> MEPHVLGAGLYWLLLPCTLLAASLLRFNALSLVYLLFLLLLPWLPGPSRHSIPGHTGRLLRALLCLSLLFLVAHLAFQICLHTVPHLDQFLGQNGSLWVKVSQHIGVTRLDLKDIFNTTRLVAPDLGVLLASSLCLGLCGRLTRKAGQSRRTQELQDDDDDDDDDDEDIDAAPAVGLKGAPALATKRRLWLASRFRVTAHWLLMTSGRTLVIVLLALAGIAHPSAFSSIYLVVFLAICTWWSCHFPLSPLGFNTLCVMVSCFGAGHLICLYCYQTPFIQDMLPPGNIWARLFGLKNFVDLPNYSSPNALVLNTKHAWPIYVSPGILLLLYYTATSLLKLHKSCPSELRKETPREDEEHELELDHLEPEPQARDATQGEMPMTTEPDLDNCTVHVLTSQSPVRQRPVRPRLAELKEMSPLHGLGHLIMDQSYVCALIAMMVWSIMYHSWLTFVLLLWACLIWTVRSRHQLAMLCSPCILLYGLTLCCLRYVWAMELPELPTTLGPVSLHQLGLEHTRYPCLDLGAMLLYLLTFWLLLRQFVKEKLLKKQKVPAALLEVTVADTEPTQTQTLLRSLGELVTGIYVKYWIYVCAGMFIVVSFAGRLVVYKIVYMFLFLLCLTLFQVYYTLWRKLLRVFWWLVVAYTMLVLIAVYTFQFQDFPTYWRNLTGFTDEQLGDLGLEQFSVSELFSSILIPGFFLLACILQLHYFHRPFMQLTDLEHVPPPGTRHPRWAHRQDAVSEAPLLEHQEEEEVFREDGQSMDGPHQATQVPEGTASKWGLVADRLLDLAASFSAVLTRIQVFVRRLLELHVFKLVALYTVWVALKEVSVMNLLLVVLWAFALPYPRFRPMASCLSTVWTCIIIVCKMLYQLKIVNPHEYSSNCTEPFPNNTNLQPLEINQSLLYRGPVDPANWFGVRKGYPNLGYIQNHLQILLLLVFEAVVYRRQEHYRRQHQQAPLPAQAVCADGTRQRLDQDLLSCLKYFINFFFYKFGLEICFLMAVNVIGQRMNFMVILHGCWLVAILTRRRREAIARLWPNYCLFLTLFLLYQYLLCLGMPPALCIDYPWRWSKAIPMNSALIKWLYLPDFFRAPNSTNLISDFLLLLCASQQWQVFSAERTEEWQRMAGINTDHLEPLRGEPNPIPNFIHCRSYLDMLKVAVFRYLFWLVLVVVFVAGATRISIFGLGYLLACFYLLLFGTTLLQKDTRAQLVLWDCLILYNVTVIISKNMLSLLSCVFVEQMQSNFCWVIQLFSLVCTVKGYYDPKEMMTRDRDCLLPVEEAGIIWDSICFFFLLLQRRIFLSHYFLHVSADLKATALQASRGFALYNAANLKSINFHRQIEEKSLAQLKRQMKRIRAKQEKYRQSQASRGQLQSKDPQDPSQEPGPDSPGGSSPPRRQWWRPWLDHATVIHSGDYFLFESDSEEEEEALPEDPRPAAQSAFQMAYQAWVTNAQTVLRQRRERARQERAEQLASGGDLNPDVEPVDVPEDEMAGRSHMMQRVLSTMQFLWVLGQATVDGLTRWLRAFTKHHRTMSDVLCAERYLLTQELLRVGEVRRGVLDQLYVGEDEATLSGPVETRDGPSTASSGLGAEEPLSSMTDDTSSPLSTGYNTRSGSEEIVTDAGDLQAGTSLHGSQELLANARTRMRTASELLLDRRLHIPELEEAERFEAQQGRTLRLLRAGYQCVAAHSELLCYFIIILNHMVTASAASLVLPVLVFLWAMLTIPRPSKRFWMTAIVFTEVMVVTKYLFQFGFFPWNSYVVLRRYENKPYFPPRILGLEKTDSYIKYDLVQLMALFFHRSQLLCYGLWDHEEDRYPKDHCRSSVKDREAKEEPEAKLESQSETGTGHPKEPVLAGTPRDHIQGKGSIRSKDVIQDPPEDLKPRHTRHISIRFRRRKETPGPKGTAVMETEHEEGEGKETTERKRPRHTQEKSKFRERMKAAGRRLQSFCVSLAQ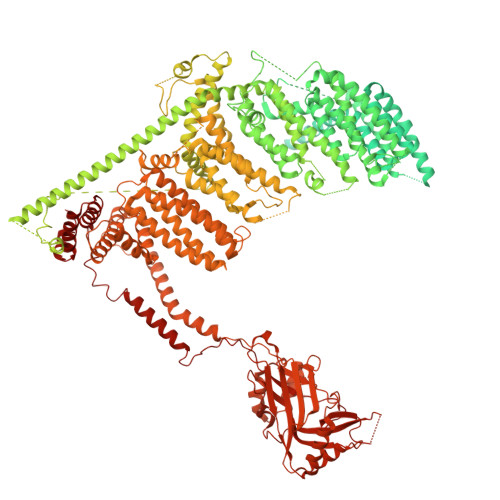SFYQPLQRFFHDILHTKYRAATDVYALMFLADIVDIIIIIFGFWAFGKHSAATDIASSLSDDQVPQAFLFMLLVQFGTMVIDRALYLRKTVLGKLAFQVVLVVAIHIWMFFILPAVTERMFSQNAVAQLWYFVKCIYFALSAYQIRCGYPTRILGNFLTKKYNHLNLFLFQGFRLVPFLVELRAVMDWVWTDTTLSLSNWMCVEDIYANIFIIKCSRETEKKYPQPKGQKKKKIVKYGMGGLIILFLIAIIWFPLLFMSLIRSVVGVVNQPIDVTVTLKLGGYEPLFTMSAQQPSIVPFTPQAYEELSQQFDPYPLAMQFISQYSPEDIVTAQIEGSSGALWRISPPSRAQMKQELYNGTADITLRFTWNFQRDLAKGGTVEYTNEKHTLELAPNSTARRQLAQLLEGRPDQSVVIPHLFPKYIRAPNGPEANPVKQLQPDEEEDYLGVRIQLRREQVGTGASGEQAGTKASDFLEWWVIELQDCKADCNLLPMVIFSDKVSPPSLGFLAGYGIVGLYVSIVLVVGKFVRGFFSEISHSIMFEELPCVDRILKLCQDIFLVRETRELELEEELYAKLIFLYRSPETMIKWTRERE>SQNMDLTIGTHRESAFYELEFGPRTIMTLANFPDDVLPLLQMESLMTFEAMAYLRCDALVELGCYDGRALEIARLLNARYLGVDLDQRAIETLRTRIEREGMSDRADTVVDDILNHTRRGASVGSRALYLLPFNLLGNFREPKRLLDSLAERSVAAVVSVFGDSAEATRVRQSYYRRCGVQGLELHTRDDGTVFTGSDGFYSRSYSRACLHALLAECGLTVVRSASNLFAHCVTVLPEGADQGFGSSAA[4x]

AZE synthases catalyse the intramolecular 4-exo-tet cyclisation of S-adenosylmethionine (SAM), yielding a highly strained heterocycle. More recently, AZE synthases have been discovered in bacteria, namely AzeJ and VioH, which are involved in the biosynthesis of azetidomonamides and vioprolides, respectively. Interestingly, they show sequence similarity to the class I methyltransferases (MT1). Each subunit adopts a classic Rossmann fold, consisting of a 7-stranded β-sheet (β3↑, β2↑, β1↑, β4↑, β5↑, β10↓, β9↑) surrounded by helices α4-6, α8-9 and α11, a topology that is typical for MT1 enzymes.

Interestingly, the Fo-Fc electron density maps reveal that MTA and AZE are bound to the active site, suggesting that the substrate has been converted via an intramolecular nucleophilic nitrogen attack on the Cγ-carbon. Intriguingly, the structural superposition of AzeJ:SAH with AzeJ:MTA:AZE only shows marginal changes of the four-membered AZE-ring in the active site (rmsd = 0.3 Å, 221 Cα-atoms), except that the nitrogen and Cγ-atoms are moved by 1.5 Å towards each other. The amine group of AZE forms hydrogen bonds with the hydroxyl group of Tyr175 and the carbonyl oxygen of Phe134. Strong cation-π interactions with Phe134 indicate a protonated state of the nitrogen atom in the AZE product. Based on the atomic insights, we propose that during cyclisation the positive charge of the sulfonium group migrates to the C-N bond and accumulates on the AZE amine. This charge distribution is stabilised by cation-π interactions with Phe134, thereby facilitating the subsequent cleavage of the Cγ-S bond, which ultimately forms the neutral molecule MTA. Moreover, the AzeJ:MTA:AZE structure provides insights into how the α-amine of SAM, protonated under physiological conditions (SAM-NH3+), can be deprotonated. Similarly as seen in AzeJ:SAH, the carboxylate of AZE forms three hydrogen bonds with Asn139, Y176 and S203. The latter two residues further coordinate with Arg172, which is additionally H-bonded to Thr193 and a water molecule.>[2x]MSVFSLKIDIADNKFFNGETSPLFSQSQAKLARQFHQKIAGYRPTPLCALDDLANLFGVKKILVKDESKRFGLNAFKMLGGAYAIAQLLCEKYHLDIETLSFEHLKNAIGEKMTFATTTDGNHGRGVAWAAQQLGQNAVIYMPKGSAQERVDAILNLGAECIVTDMNYDDTVRLTMQHAQQHGWEVVQDTAWEGYTKIPTWIMQGYATLADEAVEQ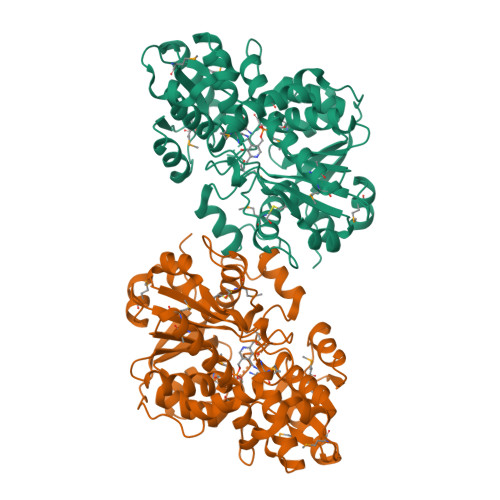MREMGVTPTHVLLQAGVGAMAGGVLGYLVDVYSPQNLHSIIVEPDKADCIYRSGVKGDIVNVGGDMATIMAGLACGEPNPLGWEILRNCATQFISCQDSVAALGMRVLGNPYGNDPRIISGESGAVGLGVLAAVHYHPQRQSLMEKLALNKDAVVLVISTEGDTDVKHYREVVWEGKHAVAP>MSHHHHHHSMDIEFMTEGPYKLPPGWRWVRLGEVCLPTERRDPTKNPSTYFVYVDISAIDSTVGKIVSPKEILGQHAPSRARKVIRSGDVIFATTRPYLKNIALVPPDLDGQICSTGFCVIRANREFAEPEFLFHLCRSDFITNQLTASKMRGTSYPAVTDNDVYNTLIPLPPLEEQRRIVAKVEALMERVREVRRLRAEAQKDTELLMQTALAEVFPHPGADLPPGWRWVRLGEVCDIIMGQSPPSSTYNFEGNGLPFFQGKADFGDLHPTPRIWCSAPQKVARPGDVLISVRAPVGSTNVAN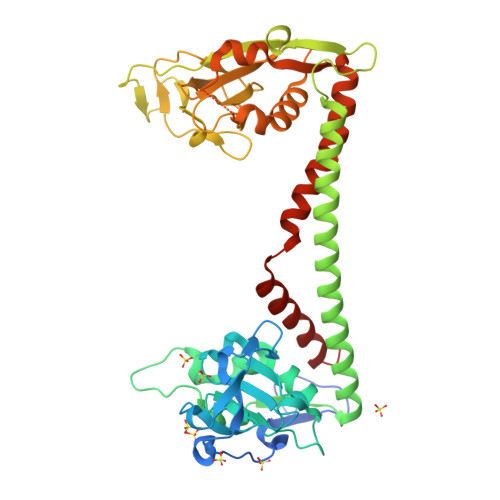LACCIGRGLAALRPRDSLERFWLLYYLHYLEPELSKMGAGSTFNAITKKDLQNVFIPLPPLEEQRRIVAYLDQIQQQVAALKRAQAETEAELKRLEQAILDKAFRGDL[2x]>[2x]SEPQDDDYLYCEMCQNFFIDSCAAHGPPTFVKDSAVDKGHP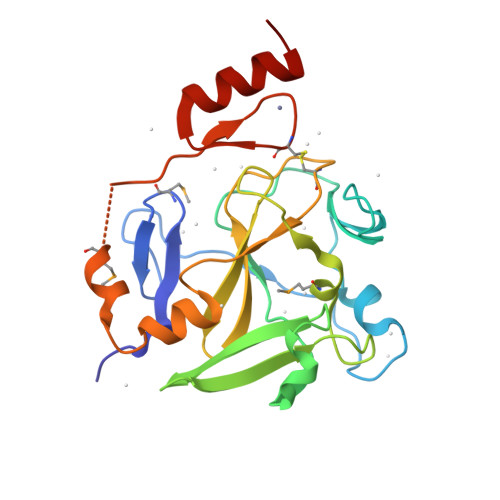NRSALSLPPGLRIGPSGIPQAGLGVWNEASDLPLGLHFGPYEGRITEDEEAANNGYSWLITKGRNCYEYVDGKDKSWANWMRYVNCARDDEEQNLVAFQYHRQIFYRTCRVIRPGCELLVWYGDEYGQELGIKWGSKWKKELMAGREPKPEIHPCPSCCLAFSSQKFLSQHVERNHSSQN>ASLT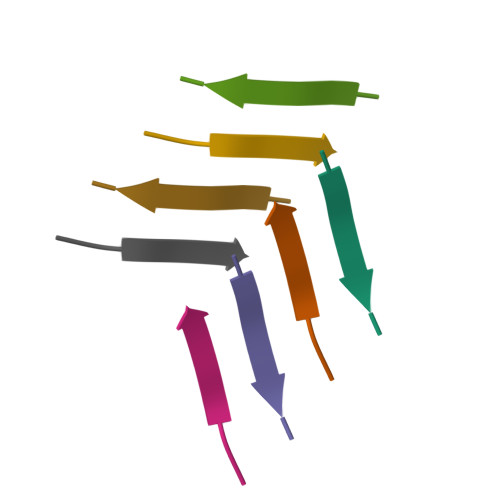VS[2x]> XMLSV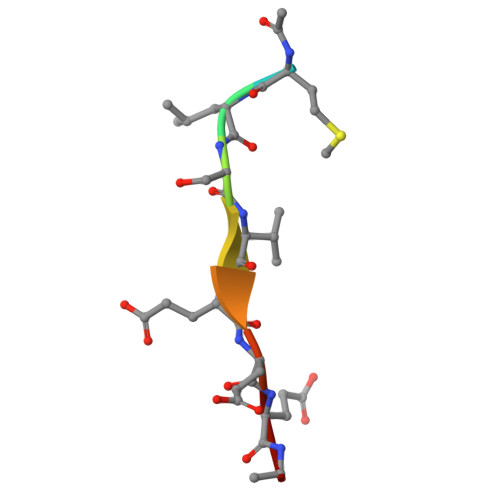EEEG>MESRVTPVAVIGMGCRLPGGINSPDKLWESLLRGDDLVTEIPPDRWDADDYYDPEPGVPGRSVSRWGGFLDDVAGFDAEFFGISEREATSIDPQQRLLLETSWEAIEHAGLDPASLAGSSTAVFTGLTHEDYLVLTTTAGGLASPYVVTGLNNSVASGRIAHTLGLHGPAMTFDTACSSGLMAVHLACRSLHDGEADLALAGGCAVLLEPHASVAASAQGMLSSTGRCHSFDADADGFVRSEGCAMVLLKRLPDALRDGNRIFAVVRGTATNQDGRTETLTMPSEDAQVAVYRAALAAAGVQPETVGVVEAHGTGTPIGDPIEYRSLARVYGAGTPCALGSAKSNMGHSTASAGTVGLIKAILSLRHGVVPPLLHFNRLPDELSDVETGLFVPQAVTPWPNGNDHTPKRVAVSSFGMSGTNVHAIVEEAPAEASAPESSPGDAEVGPRLFMLSSTSSDALRQTARQLATWVEEHQDCVAASDLAYTLARGRAHRPVRTAVVAANLPELVEGLREVADGDALYDAAVGHGDRGPVWVFSGQGSQWAAMGTQLLASEPVFAATIAKLEPVIAAESGFSVTEAITAQQTVTGIDKVQPAVFAVQVALAATMEQTYGVRPGAVVGHSMGESAAAVVAGALSLEDAARVICRRSKLMTRIAGAGAMGSVELPAKQVNSELMARGIDDVVVSVVASPQSTVIGGTSDTVRDLIARWEQRDVMAREVAVDVASHSPQVDPILDDLAAALADIAPMTPKVPYYSATLFDPREQPVCDGAYWVDNLRNTVQFAAAVQAAMEDGYRVFAELSPHPLLTHAVEQTGRSLDMSVAALAGMRREQPLPHGLRGLLTELHRAGAALDYSALYPAGRLVDAPLPAWTHARLFIDDDGQEQRAQGACTITVHPLLGSHVRLTEEPERHVWQGDVGTSVLSWLSDHQVHNVAALPGAAYCEMALAAAAEVFGEAAEVRDITFEQMLLLDEQTPIDAVASIDAPGVVNFTVETNRDGETTRHATAALRAAEDDCPPPGYDITALLQAHPHAVNGTAMRESFAERGVTLGAAFGGLTTAHTAEAGAATVLAEVALPASIRFQQGAYRIHPALLDACFQSVGAGVQAGTATGGLLLPLGVRSLRAYGPTRNARYCYTRLTKAFNDGTRGGEADLDVLDEHGTVLLAVRGLRMGTGTSERDERDRLVSERLLTLGWQQRALPEVGDGEAGSWLLIDTSNAVDTPDMLASTLTDALKSHGPQGTECASLSWSVQDTPPNDQAGLEKLGSQLRGRDGVVIVYGPRVGDPDEHSLLAGREQVRHLVRITRELAEFEGELPRLFVVTRQAQIVKPHDSGERANLEQAGLRGLLRVISSEHPMLRTTLIDVDEHTDVERVAQQLLSGSEEDETAWRNGDWYVARLTPSPLGHEERRTAVLDPDHDGMRVQVRRPGDLQTLEFVASDRVPPGPGQIEVAVSMSSINFADVLIAFGRFPIIDDREPQLGMDFVGVVTAVGEGVTGHQVGDRVGGFSEGGCWRTFLTCDANLAVTLPPGLTDEQAITAATAHATAWYGLNDLAQIKAGDKVLIHSATGGVGQAAISIARAKGAEIFATAGNPAKRAMLRDMGVEHVYDSRSVEFAEQIRRDTDGYGVDIVLNSLTGAAQRAGLELLAFGGRFVEIGKADVYGNTRLGLFPFRRGLTFYYLDLALMSVTQPDRVRELLATVFKLTADGVLTAPQCTHYPLAEAADAIRAMSNAEHTGKLVLDVPRSGRRSVAVTPEQAPLYRRDGSYIITGGLGGLGLFFASKLAAAGCGRIVLTARSQPNPKARQTIEGLRAAGADIVVECGNIAEPDTADRLVSAATATGLPLRGVLHSAAVVEDATLTNITDELIDRDWSPKVFGSWNLHRATLGQPLDWFCLFSSGAALLGSPGQGAYAAANSWVDVFAHWRRAQGLPVSAIAWGAWGEVGRATFLAEGGEIMITPEEGAYAFETLVRHDRAYSGYIPILGAPWLADLVRRSPWGEMFASTGQRSRGPSKFRMELLSLPQDEWAGRLRRLLVEQASVILRRTIDADRSFIEYGLDSLGMLEMRTHVETETGIRLTPKVIATNNTARALAQYLADTLAEEQAAAPAASKLAAALEHHHHHH[2x]

As exemplified by isoniazid, which targets the enoylreductase in mycolic acid biosynthesis, mycocerosic acid synthase (MAS) offers a potential drug target by producing part of phthiocerol dimycocerosate (PDIM), a key component of the cell envelope. MAS, a fully reducing iterative type I polyketide synthase (PKS), is composed of six domains that together catalyze the elongation of n-C6-C20 fatty acids to prepare mycocerosic acid. Using a combination of dual covalent crosslinking and cryo-EM analyses, we elucidate the structure of mycocerosic acid synthase from Mycobacterium tuberculosis trapped in two distinct catalytic states during its iterative cycle. These structures reveal domain architecture of the acyl carrier protein mediating condensation and dehydration through dual site-selective crosslinking of the acyl carrier protein with the ketosynthase and dehydratase domains.

We also obtained a map of the modifying compartment DH-ΨKR-ER-KR-ACP (3.74 Å) from the same dataset. Complex C demonstrated the modifying compartment (DH-ΨKR-ER-KR), with ACP crosslinked with DH through 1. In this complex, 1 covalently crosslinks the ACP to the active site His929 of the DH. In contrast to the extensive interactions between the highly negatively charged AcpP (helices 2 and 3) and a positively charged patch of FabA, the ACP in MAS shows only limited interactions with the DH domain between Thr2072 of helix 2 of ACP and Asn933 of DH. Arg2045, Thr2046, and Tyr2056 (ACP loop 1) interact with Ser1187 and Glu2000 of inter-domain linkers (L2 and L5). Unlike the shunt product in complex B, there is no probe observed in the uncrosslinked DH of the opposite protomer, indicating that the reactivity between crosslinker 1 and DH is facilitated by ACP binding. Unlike the narrow and well-defined FabA active site, MAS-DH features a deep binding tunnel to accommodate the long, branched-chain acyl intermediates. Surprisingly, while the E. coli type II DH regulates the substrate specificity via gating residues, we observe a major domain rotation of the crosslinked DH in comparison to the apo-DHs in MAS complex A and MAS-like PKS modifying compartment. In the DH apo form the active site entrance resides underneath the ΨKR • KR domains, providing no access for ACP binding. In complex C, the DH translates and rotates away from the ΨKR • KR to enable access to the ACP.>MNQSVSSLPEKDIQYQLHPYTNARLHQELGPLIIERGEGIYVYDDQGKGYIEAMAGLWSAALGFSNQRLIKAAEQQFNTLPFYHLFSHKSHRPSIELAEKLIEMAPVPMSKVFFTNSGSEANDTVVKMVWYLNNALGKPAKKKFISRVNGYHGITVASASLTGLPGNQRGFDLPLPGFLHVGCPHHYRFALAGESEEHFADRLAVELEQKILAEGPETIAAFIGEPLMGAGGVIVPPRTYWEKIQKVCRKYDILVIADEVICGFGRTGQMFGSQTFGIQPDIMVLSKQLSSSYQPIAAILINAPVFEGIADQSQ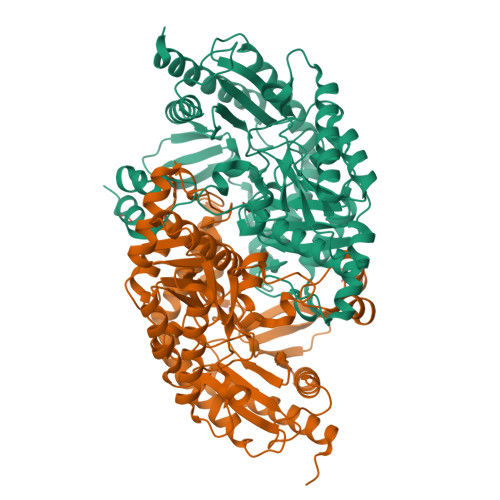ALGALGHGFTGSGHPVATAVALENLKIIEEESLVEHAAQMGQLLRSGLQHFIDHPLVGEIRGCGLIAAVELVGDRVSKAPYQALGTLGRYMAGRAQEHGMITRAMGDAVAFCPPLIVNEQEVGMIVERFARALDDTTQWVGPGGHHHHHH[2x]>[2x]GHMSGEAPLTATVDGIIQPMLKAYRIPGMAVAVLKDGKAHYFNYGVANRESGQRVSEQTLFEIGS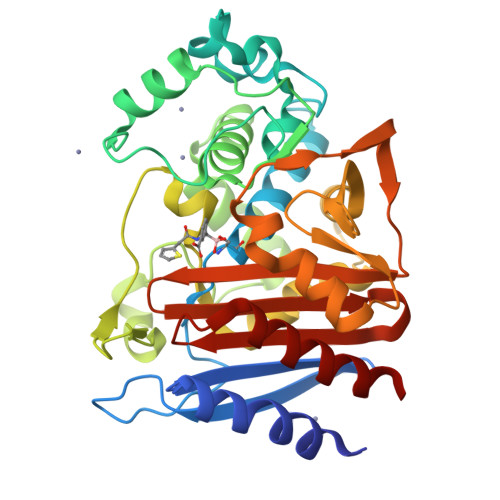VSKTLTATLGAYAAVKGGFELDDKVSQHAPWLKGSAFDGVTMAELATYSAGGLPLQFPDEVDSNDKMQTYYRSWSPVYPAGTHRQYSNPSIGLFGHLAANSLGQPFEQLMSQTLLPKLGLHHTYIQVPESAMANYAYGYSKEDKPIRATPGVLAAEAYGIKTGSADLLKFVEANMGYQGDAALKSAIALTHTGFHSVGEMTQGLGWESYDYPVTEQVLLAGNSPAVSFQANPVTRFAVPKAMGEQRLYNKTGSTGGFGAYVAFVPARGIAIVMLANRNYPIEARVKAAHAILSQLAE>[6x]MAHHHHHHVGTGSNDDDDKSPDPMRAIWTGSIAFGLVNVPVKVYSATADHDIRFHQVHAKDNGRIRYKRVCEACGEVVDYRDLARAYESGDGQMVAITDDDIASLPEERSREIEVLEFVPAADVDPMMFDRSYFLEPDSKSSKSYVLLAKTLAETDRMAIVHFTLRNKTRLAALRVKDFGK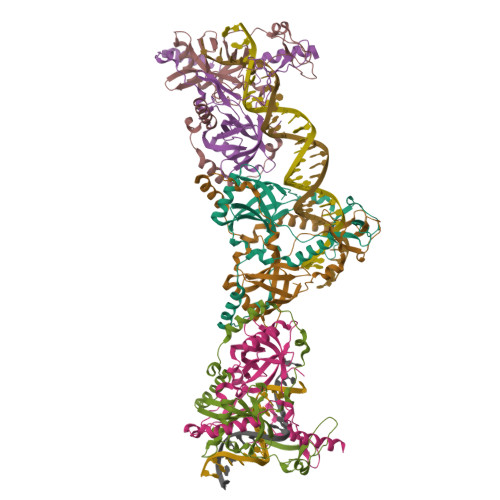REVMMVHTLLWPDEIRDPDFPVLDQKVEIKPAELKMAGQVVDSMADDFNPDRYHDTYQEQLQELIDTKLEGGQAFTAEDQPRLLDEPEDVSDLLAKLEASVKARSKANSNVPTPP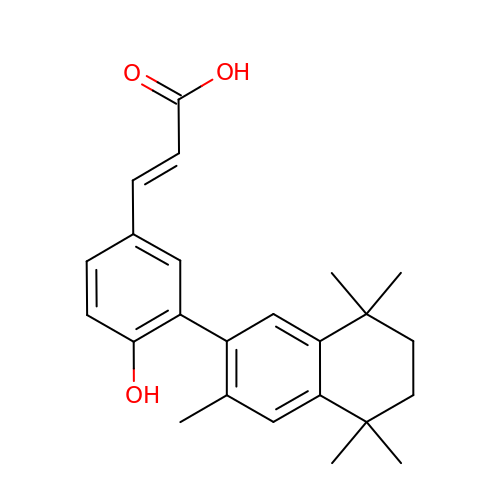(2E)-3-[4-hydroxy-3-(3,5,5,8,8-pentamethyl-5,6,7,8-tetrahydronaphthalen-2-yl)phenyl]prop-2-enoic acid | C24 H28 O3 | DYLLZSVPAUUSSB-VQHVLOKHSA-N>[4x]EFRHDSRKIPKVGHTFFQKPESCPPVPGGSMKLDIGIINENQRVSMSRNIESRSTSPWNYTVTWDPNRYPSEVVQAQCRNLGCINAQGKEDISMNSVPIQQETLV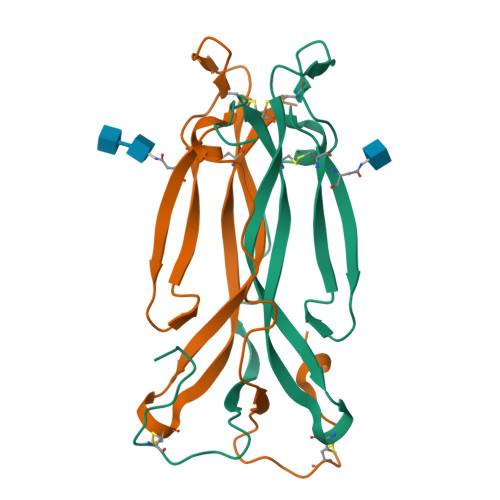VRRKHQGCSVSFQLEKVLVTVGCTCVTPVIHHVQ In order to shed light on this fundamental mechanism, we studied S. aureus FapR (SaFapR) a transcription factor that senses the levels of malonyl-CoA, a key intermediate in fatty acid biosynthesis, and modulates the expression of genes involved in fatty acid and phospholipid biosynthesis. FapR has been shown to globally repress the expression of the genes from the fap regulon encoding the soluble FASII system as well as two key enzymes that interface this pathway with the synthesis of phospholipid molecules. Like most transcriptional regulators in bacteria, FapR is a homodimeric repressor. Each protomer consists of a N-terminal DNA-binding domain (DBD) harboring a classical helix-turn-helix motif connected through a linker α-helix (αL) to a C-terminal effector-binding domain (EBD).

The crystal structure of full-length SaFapR in the absence of ligands has been obtained in two different crystal forms. Interestingly, in three out of four crystallographically independent protomers the repressor has the same non-productive quaternary arrangement as observed in the structure of malonyl-CoA-bound SaFapR, with helix αL bound to the lateral face of the EBD, strongly suggesting that this compact structure likely represents a conformation of the protein in solution. However, the helix-turn-helix motifs display high temperature factors or even partial disorder, and are engaged in extensive crystal contacts, suggesting the coexistence of alternative conformational states in solution characterized by flexible DBDs. In that sense, in one protomer of the crystal form 2 both helix αL and its associated DBD are highly flexible and could not be modeled, suggesting a marginal stability of the observed quaternary arrangement. Moreover, the first visible residues of this same monomer (positions 72–77, connecting helix αL with the first β-strand of the EBD) adopt a conformation that differs from that observed in the other ligand-free or malonyl-CoA-bound protomers, but resembles that found for one subunit of the asymmetric DNA-bound form of the repressor. Similarly to other homodimeric proteins studied by single-molecule or NMR relaxation approaches, our crystallographic studies suggest that the two conformational states of SaFapR (i.e. with EBD-bound or EBD-detached DBDs) can be populated in the ligand-free repressor species.

>[2x]MRGETLKLKKDKRREAIRQQIDSNPFITDHELSDLFQVSIQTIRLDRTYLNIPELRKRIKLVAEKNYDQISSIEEQEFIGDLIQVNPNVKAQSILDITSDSVFHKTGIARGHVLFAQANSLCVALIKQPTVLTHESSIQFIEKVKLNDTVRAEARVVNQTAKHYYVEVKSYVKHTLVFKGNFKMFYDKRG> MAHNTELLPIELDTLVGKGRFAEVYKAKLKQNTSEQFETVAVKIFPYEEYASWKTEKDIFSDINLKHENILQFLTAEERKTELGKQYWLITAFHAKGNLQEYLTRHVISWEDLRKLGSSLARGIAHLHSDHTPCGRPKMPIVHRDLKSSNILVKNDLTCCLCDFGLSLRLDPTLSVDDLANSGQVGTARYMAPEVLASAMNLENVESFKQTDVYSMALVLWEMTSRCNAVGEVKDYEPPFGSKVREHPCVASMADNVLADAGRPEIPSFWLNHQGIQMVCETLTECWDHDPEARLTAQCVAER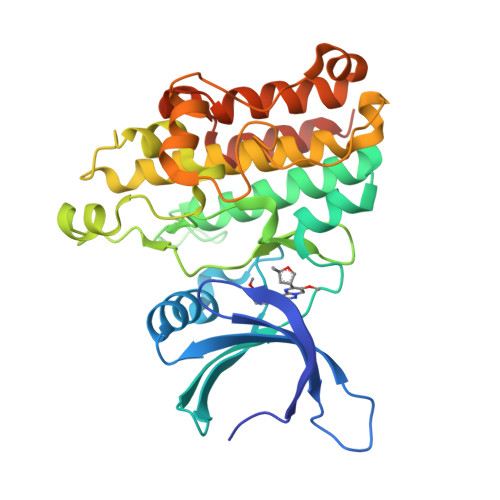FSELEHLDRLSGLEHHHHHH> ALWQFNGMIKCKIPSSEPLLDFNNYGCYCGLGGSGTPVDDLDRCCQTHDNCYMQAMKLDSCKVLVDNPYTNNYSYSCSNNEITCSSENNACEAF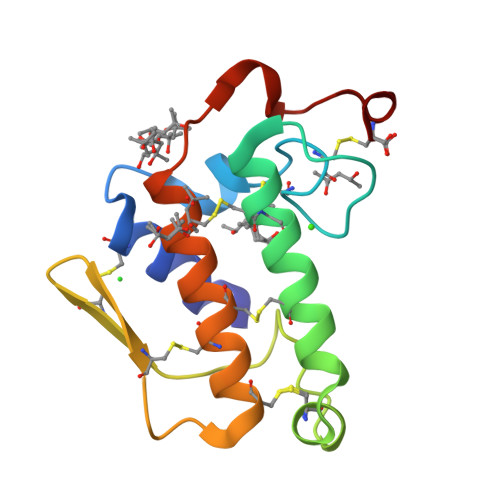ICNCDRNAAICFSKVPYNKEHKNLDMMNC> ISEFGSEPIDPSKLEFARALYDFVPENPEMEVALKKGDLMAILSKKDPLGRDSDWW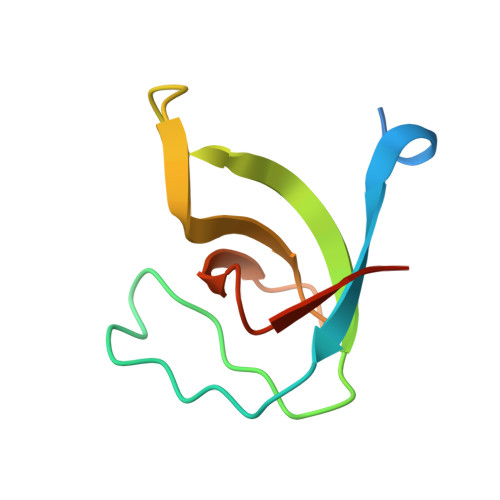KVRTKNGNIGYIPYNYIEIIKRRK>[2x]GPLPAHDASKVRASGPGLNASGIPASLPVEFTIDARDAGEGLLTVQILDPEGKPKKANIRDNGDGTYTVSYLPDMSGRYTITIKYGGDEIPYSPFRIHALPT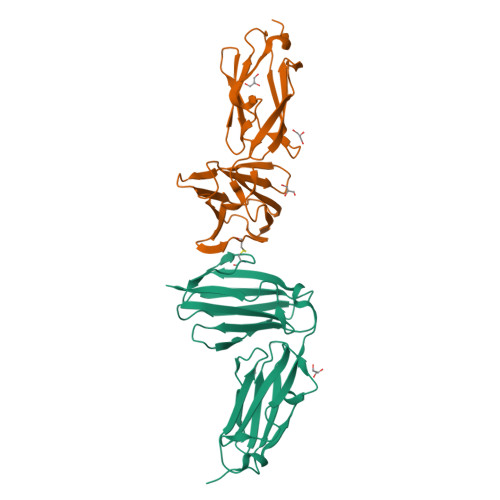GDASKCLVTVSIGGHGLGACLGPRIQIGQETVITVDAKAAGERKVTCTVSTPDGAELDVDVVENHDGTFDIYYTAPEPGKYVITIRFGGEHIPNSPFHVLATE>MLNQELELSLNMAFARAREHRHEFMTVEHLLLALLSNPSAREALEACSVDLVALRQELEAFIEQTTPVLPASEEERDTQPTLSFQRVLQRAVFHVQSSGRNEVTGANVLVAIFSE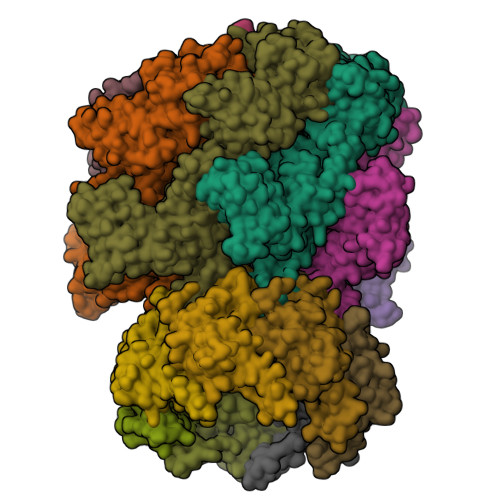QESQAAYLLRKHEVSRLDVVNFISHGTRKDEPTQSSDPGSQPNSEEQAGGEERTENFTTNLNQLARVGGIDPLIGREKELERAIQVLCRRRKNNPLLVGESGVGKTAIAEGLAWRIVQGDVPEVMADCTIYSLDIGSLLAGTKYRGDFEKRFKALLKQLEQDTNSILFIDEIHTIIGAGAASGGQVDAANLIKPLLSSGKIRVIGSTTYQEFSNIFEKDRALARRFQKIDITEPSIEETVQIINGLKPKYEAHHDVRYTAKAVRAAVELAVKYINDRHLPDKAIDVIDEAGARARLMPVSKRKKTVNVADIESVVARIARIPEKSVSQSDRDTLKNLGDRLKMLVFGQDKAIEALTEAIKMARAGLGHEHKPVGSFLFAGPTGVGKTEVTVQLSKALGIELLRFDMSEYMERHTVSRLIGAPPGYVGFDQGGLLTDAVIKHPHAVLLLDEIEKAHPDVFNILLQVMDNGTLTDNNGRKADFRNVVLVMTTNAGVRETERKSIGLIHQDNSTDAMEEIKKIFTPEFRNRLDNIIWFDHLSTDVIHQVVDKFIVELQVQLDQKGVSLEVSQEARNWLAEKGYDRAMGARPMARVIQDNLKKPLANELLFGSLVDGGQVTVALDKEKNELTYGFQSAQKHKAEAAH[6x];>ALVPMVIEQTSRGERSFDIYSRLLKERVIFLTGQVEDHMANLIVAQMLFLEAENPEKDIYLYINSPGGVITAGMSIYDTMQFIKPDVSTICMGQAASMGAFLLTAGAKGKRFCLPNSRVMIHQPLGGYQGQATDIEIHAREILKVKGRMNELMALHTGQSLEQIERDTERDRFLSAPEAVEYGLVDSILTHRNRSHHHHHH[7x];> MGKTNDWLDFDQLAEEKVRDALKPPSMYKVILVNDDYTPMEFVIDVLQKFFSYDVERATQLMLAVHYQGKAICGVFTAEVAETKVAMVNKYARENEHPLLCTLEKA>ATVGPRVIVVGAGMSGISAAKRLSEAGITDLLILEATDHIGGRMHKTNFAGINVELGANWVEGVNGGKMNPIWPIVNSTLKLRNFRSDFDYLAQNVYKEDGGVYDEDYVQKRIELADSVEEMGEKLSATLHASGRDDMSILAMQRLNEHQPNGPATPVDMVVDYYKFDYEFAEPPRV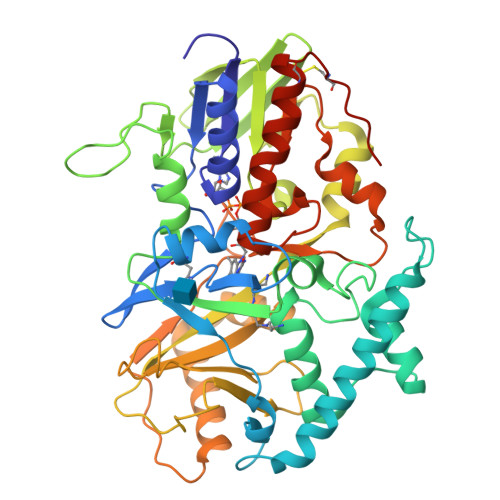TSLQNTVPLATFSDFGDDVYFVADQRGYEAVVYYLAGQYLKTDDKSGKIVDPRLQLNKVVREIKYSPGGVTVKTEDNSVYSADYVMVSASLGVLQSDLIQFKPKLPTWKVRAIYQFDMAVYTMIFLKFPRKFWPEGKGREFFLYASSRRGYYGVWQEFEKQYPDANVLLVTVTDEESRRIEQQSDEQTKAEIMQVLRKMFPGKDVPDATDILVPRWWSDRFYKGTFSNWPVGVNRYEYDQLRAPVGRVYFTGEHTSEHYNGYVHGAYLSGIDSAEILINCAQKKMCKYHVQGKYDHHHHHH[2x]> AEESRKRLRFARLSEHATAPTKGSERAAGYDLYSAYDYTVLPMEKAIVKTDIQIALPS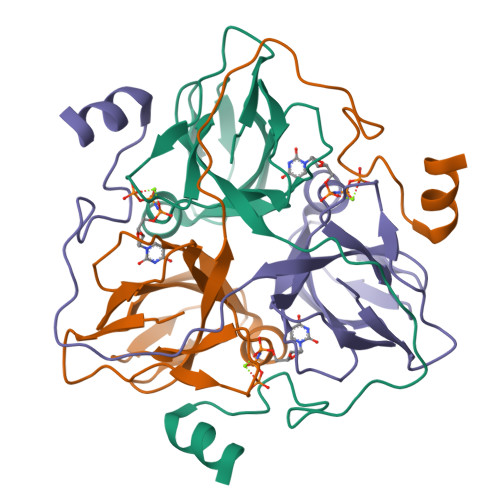GCYGRVAPRSGLAAKHFIDVGAGVIDEDYRGNVGVVLFNFGKEKFEVKKGDRIAQLICERIFYPEIEEVQVLDDTERGSGGFGSTGTNLEHHHHHHH> HHHHHHRQYNLVTRESLPQALRRIEEAKRIALDTETTGLQIYLPGFELVGLAVAVSPEEAYYFPYAHRDFAGLRYQPENLSREDLLRVLELAFQRSVVYHNAAYDRQVLYRTLGIPFERSYGNDTMIALHLMDENHSNSLKEWSKTLLGLEESMAVPELPSLTDVELVDTVNKSGRKYKKKVHKLAPDWLDRLKTAFLSVHNGGVSFAALHKLVAQAFNTLKARGILYYPGSFPVDFRYFHVHLAHIYALDDAMNTLALWEHVEIFLQLHPQLERLYLDIELPVNDIMTRASARGVLVDRSVIERIEADLQAKLEERE

The structure of PolI_G20c was solved with the aid of the structure of an exonuclease termed ExnV1, which was determined in parallel in this work and originates from an Icelandic virus metagenome collected from several hot springs in Iceland. The gene coding for ExnV1 may be part of a truncated gene that originally encoded a DNA polymerase I. A novel structural motif, SβαR, that was not previously associated with DNA polymerases I was identified in the solved structures of ExnV1 and PolI_G20c. Residues 152–185 are missing in chain B of PolI_G20c; however, the residues corresponding to those in ExnV1 are present and from the sequence alignment it is interpreted that PolI_G20c also resembles ExnV1 in this area, which is part of a novel structure motif (SβαR) that is discussed further below. The major difference between the two proteins is that ExnV1 only comprises the smaller 3′–5′ exonuclease, whereas PolI_G20c also includes the larger palm domain that is responsible for the polymerase activity. The SβαR structural motif consists of two β-strands followed by two α-helices that are connected to each other via a short β-strand.

The gene coding for ExnV1 originates from a metagenome collected within the Virus-X project. It has a length of 942 bp (corresponding to 314 residues), and sequence comparison using BlastP and the CDD revealed that ExnV1 only contains the putative 3′–5′ exonuclease domain typical of DNA polymerases I, indicating that ExnV1 may be a truncated DNA polymerase I. The crystal structure of ExnV1 contained one polypeptide chain and the overall structure was determined to 2.19 Å resolution using the co-crystallized terbium compound. The structure of PolI_G20c consists of two polypeptide chains, A and B, that could possibly be arranged as a dimer according to PISA structure analysis in CCP4mg. ExnV1 corresponds to the first 315 residues of PolI_G20c, and superposition of ExnV1 on PolI_G20c (with an r.m.s.d. of 1.01 Å over 236 residues) shows that the structures of the two proteins match each other very well. The major difference between the Klenow fragment, PolI_G20c and ExnV1 is that the latter two have a separate structure towards the end of the 3′–5′ exonuclease domain, corresponding to residues 157–222 in ExnV1 and 158–223 in PolI_G20c. This specific structural motif, termed SβαR, consists of two rather long β-strands in ExnV1, followed by two α-helices corresponding to α-helices 7 and 8, with a very short β-strand 10 between them. ExnV1 was also investigated using the DALI server against the PDB. The search generated 13 matches with a Z-value above 20 and all of these models are Klenow fragments of DNA polymerase I from E. coli.phenylmethanethiol | C7 H8 S | 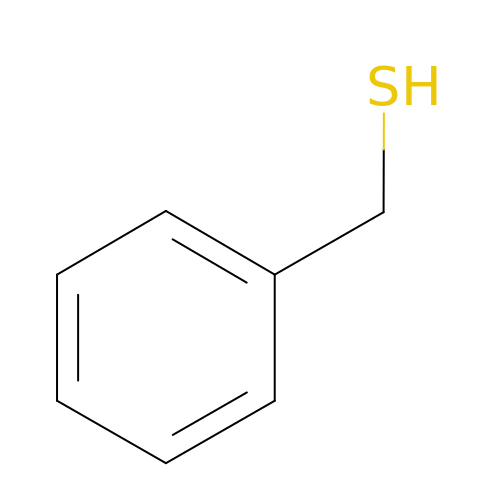UENWRTRMUIOCKN-UHFFFAOYSA-N> GPLGSMSTVGSAHNVRVLGSGETTVVLGHGFGTDQSVWKQ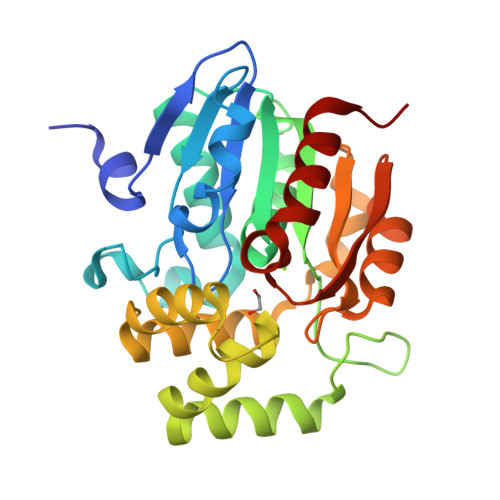LVPYLTDEYRVLLYDNMGAGTTNPDCYDFERYSSLEGHSNDLIAILDDFHVTKCIYVGHSLSSMAAAVSSIFRPDLFRKVVMISATPRITNTEDYYGGFEQEEINQMNTAMEENFKTMMMGFAPIVVGGDLESDAIQEFSRTLFNMRPDIALSICRMISGLDLRPYLGLIVVPCHIIQSSKDMLVPVAVAEYLHKNLGGKSVVELIPTEGHLPHLSAPELTIPVLVRHIKHDIA Cthe_2751_is a 15.8 kDa singleton from an anaerobic, hyperthermophile Clostridium thermocellum, with an unknown function. Therefore, based on primary sequence analysis, Cthe_2751 is a non-Pfam singleton with an unknown function. Each monomer is made up of 8 α-helices arranged in a spiral pattern around a vertical axis that runs through the centre of the protein. The structure reveals an all α-helical topology similar to those observed for nucleic acid processing proteins.

Cthe_2751 crystallized as a dimer in 3 different crystal forms. Superimposition of the dimers crystallized in different space groups revealed no obvious differences in the position of the Cα atoms suggesting an identical mode of dimerization in all the 3 crystal forms. To find out if there is a difference in the packing arrangement of the dimers in the 3 crystal forms and to quantify it, a computer program was compiled and a calculation was performed to analyze the inter-dimer distances of 2 neighbouring dimers for all 3 space groups. As expected, the inter-dimer distance between 2 closest dimers in space groups C2221 and P4122 is relatively similar when compared to that of the distance between dimers of space groups P212121 and C2221 or P212121 and P4122, where there is almost no recognizable co-relationship. This result further supports the inferences of crystal packing analysis where we saw that the dimers rotate less than 3° along the C axes during the transformation from P4122 to C2221 resulting in only a minor change in crystal packing. A mathematical calculation performed on the dimers of Cthe_2751 crystallized in different space groups corroborated the findings of the crystal packing analysis of molecules packed in different space groups.

>MTSLRDLIPKHKFDNSTIDQLCKLIDNEIEPIIFDLLKWLQDYNWPIAKDILPVVVLHQSIAMPHILTILQGNDIMWKYWVIKLMIPYLIYPNKQLVKSELERLSSLEIINEDIREIVNLSKDYLHFYYPDKHN[2x]> WTKEENQSVVVDFLLPTGVYLNFPVSRNANLSTIKQLLWHRAQYEPLFHMLSGPEAYVFTCINQTAEQQELEDEQRRLCDVQPFLPVLRLVAREGDRVKKLINSQISLLIGKGLHEFDSLCDPEVNDFRAKMCQFCEEAAARR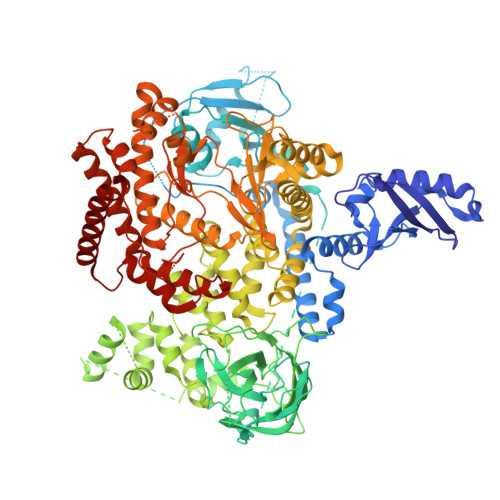QQLGWEAWLQYSFPLQLEPSAQTWGPGTLRLPNRALLVNVKFEGSEESFTFQVSTKDVPLALMACALRKKATVFRQPLVEQPEDYTLQVNGRHEYLYGSYPLCQFQYICSCLHSGLTPHLTMVHSSSILAMRDEQSNPAPQVQKPRAKPPPIPAKKPSSVSLWSLEQPFRIELIQGSKVNADERMKLVVQAGLFHGNEMLCKTVSSSEVSVCSEPVWKQRLEFDINICDLPRMARLCFALYAVIEKAKKARSTKKKSKKADCPIAWANLMLFDYKDQLKTGERCLYMWPSVPDEKGELLNPTGTVRSNPNTDSAAALLICLPEVAPHPVYYPALEKILELGRHSECVHVTEEEQLQLREILERRGSGELYEHEKDLVWKLRHEVQEHFPEALARLLLVTKWNKHEDVAQMLYLLCSWPELPVLSALELLDFSFPDCHVGSFAIKSLRKLTDDELFQYLLQLVQVLKYESYLDCELTKFLLDRALANRKIGHFLFWHLRSEMHVPSVALRFGLILEAYCRGSTHHMKVLMKQGEALSKLKALNDFVKLSSQKTPKPQTKELMHLCMRQEAYLEALSHLQSPLDPSTLLAEVCVEQCTFMDSKMKPLWIMYSNEEAGSGGSVGIIFKNGDDLRQDMLTLQMIQLMDVLWKQEGLDLRMTPYGCLPTGDRTGLIEVVLRSDTIANIQLNKSNMAATAAFNKDALLNWLKSKNPGEALDRAIEEFTLSCAGYCVATYVLGIGDRHSDNIMIRESGQLFHIDFGHFLGNFKTKFGINRERVPFILTYDFVHVIQQGKTNNSEKFERFRGYCERAYTILRRHGLLFLHLFALMRAAGLPELSCSKDIQYLKDSLALGKTEEEALKHFRVKFNEALRESWKTKV> MELKNKKWTDEEFHKQREEVLQQWPTGKEVDLQEAVDYLKKIPAEKNFAEKLVLAKKKGITMAQPRAGVALLDEHIELLRYLQDEGGADFLPSTIDAYTRQNRYDECENGIKESEKAG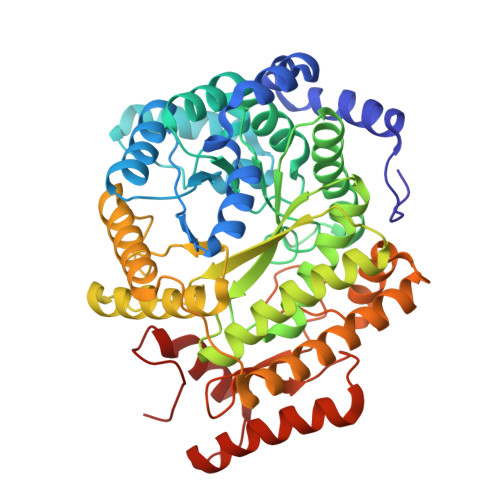RSLLNGFPGVNFGVKGCRKVLEAVNLPLQARHGTPDSRLLAEIIHAGGWTSNEGGGISYNVPYAKNVTIEKSLLDWQYCDRLVGFYEEQGVHINREPFGPLTGTLVPPSMSNAVGITEALLAAEQGVKNITVGYGECGNMIQDIAALRCLEEQTNEYLKAYGYNDVFVTTVFHQWMGGFPQDESKAFGVIVTATTIAALAGATKVIVKTPHEAIGIPTKEANAAGIKATKMALNMLEGQRMPMSKELETEMAVIKAETKCILDKMFELGKGDLAIGTVKAFETGVMDIPFGPSKYNAGKMMPVRDNLGCVRYLEFGNVPFTEEIKNYNRERLQERAKFEGRDVSFQMVIDDIFAVGKGRLIGRPE> GPGIQVKALYDYDAQTGD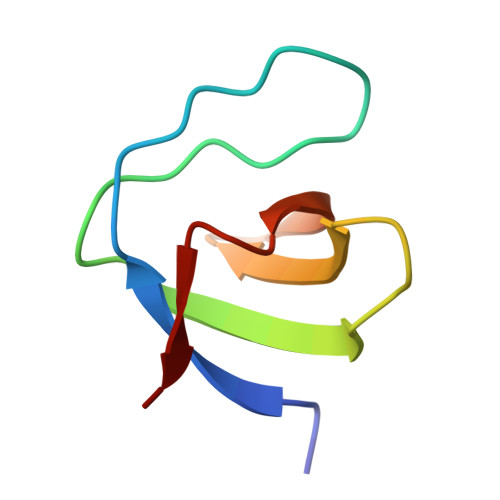ELTFKEGDTIIVHQKDPAGWWEGELNGKRGWVPANYVQDI>GSHMAS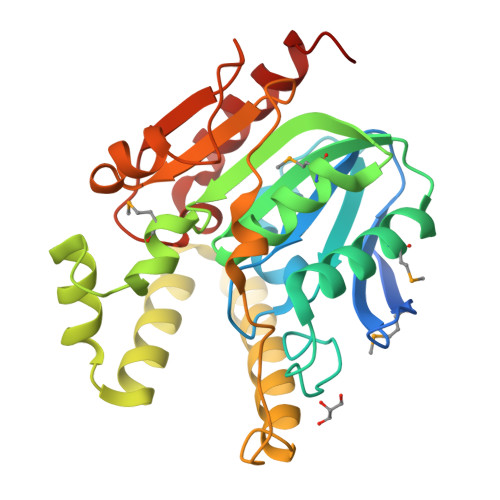MTGGQQMGRGSMAALNKEMVNTLLGPIYTCHREGNPCFVFLSGAGFFSTADNFANIIDKLPDSIGILTIDAPNSGYSPVSNQANVGLRDWVNAILMIFEHFKFQSYLLCVHSIGGFAALQIMNQSSKACLGFIGLEPTTVMIYRAGFSSDLYPQLALRRQKLKTAADRLNYLKDLSRSHFSSQQFKQLWRGYDYCQRQLNDVQSLPDFKIRLALGEEDFKTGISEKIPSIVFSESFREKEYLESEYLNKHTQTKLILCGQHHYLHWSETNSILEKVEQLLSNHEKL[2x]> WELTILHTNDVHSRLEQTSEDSSKCVDASRCMGGVARLFTKVQQIRRAEPNVLLLDAGDQYQGTIWFTVYKGAEVAHFMNALRYDAMALGNHEFDNGVEGLIEPLLKEAKFPILSANIKAKGPLASQISGLYLPYKVLPVGDEVVGIVGYTSKETPFLSNPGTNLVFEDEITALQPEVDKLKTLNVNKIIALGHSGFEMDKLIAQKVRGVDVVVGGHSNTFLYTGNPPSKEVPAGKYPFIVTSDDGRKVPVVQAYAFGKYLGYLKIEFDERGNVISSHGNPILLDSSIPEDPSIKADINKWRI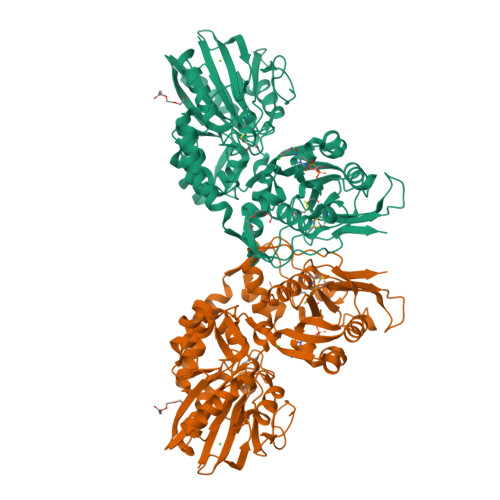KLDDYSTQELGKTIVYLDGSSQSCRFRECNMGNLICDAMINNNLRHTDEMFWNHVSMCILNGGGIRSPIDERNDGTITWENLAAVLPFGGTFDLVQLKGSTLKKAFEHSVHRYGQSTGEFLQVGGIHVVYDLSRKPGDRVVKLDVLCTSCRVPSYDPLKMDEVYKVILPNFLANGGDGFQMIKDELLRHDSGDQDINVVSTYISKMKVIYPAVEGRIKFSGGGGAGGGGGTDDDDKWSHPQFEK>[4x]MAEMLVKSKVKEFVKSVDPEMRVSPEFYDALEAEVKALVEKAIKRAQAEGRKTLYARHV

Histones are important chromatin-organizing proteins in eukaryotes and archaea. They form superhelical structures around which DNA is wrapped. Alongside nucleosomal histones, we identify a second major prokaryotic histone family, termed α3 histones, with representatives in almost all archaeal phyla and several bacteria. Face-to-face (FtF) histones make up the largest subcategory of α3 histones (83%) and are, after nucleosomal histones, the largest group of histones in prokaryotes.

FtF histones are defined by their predicted tetramer structure. In the tetramer, two dimers interact in a manner similar to nucleosomal histones, via their α3 helices and the last  ~8 amino acids of their α2 helix. Unlike nucleosomal histones, both sides of the dimer interact, forming a torus. To confirm the predicted tetramer structure of FtF-histones, we purified and crystallized the FtF histone from Thermococcus kodakarensis, which we refer to as HTkC. The asymmetric unit contains two histone dimers, that assemble into a torus-shaped tetramer. With a Cα RMSD of 0.652 Å, the HTkC crystal structure is virtually identical to the AlphaFold prediction, highlighting AlphaFold’s accuracy in predicting histone structures. For face-to-face (FtF) histones, which form the largest subgroup of α3 histones, we confirmed their unique quaternary structure by crystallography. The FtF histone, HTkC, in T. kodakarensis is part of the top 7% of the highest expressed genes, with an expression level that is 34 times lower than that of hypernucleosome histone HTkA. The α3 family compromises five histone categories, each of which is likely related to a different function as they differ in predicted quaternary structure and the presence of additional domains: face-to-face, bacterial dimer, ZZ, Rab GTPase, and phage histones. These categories are discussed in more detail below. α3 histones are defined by a truncated α3 helix, which, compared to the 10 amino acid long nucleosomal α3 helix, consists only of 3 to 4 amino acids. Residues R47, T49, and D54 form an RxTxxxxD motif which is also present in nucleosomal histones from archaea.>RSPRLVGADMPCSGRVEVKHADTWRSVCDSDFSLHAANVLCRELNCGDAISLSVGDHFGKGNGLTWAEKFQCEGSETHLALC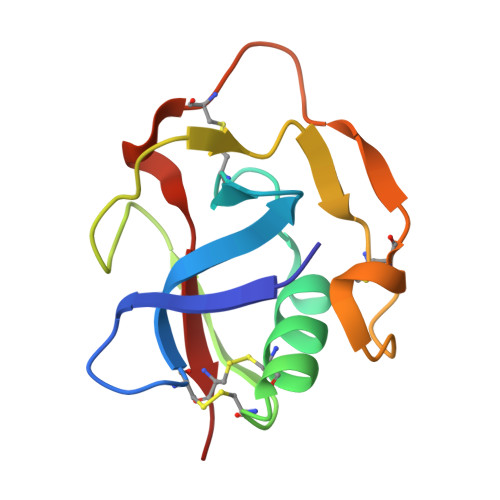PIVQHPEDTCIHSREVGVVCST[2x]> MSVKASGGSSLARPQLYQTVPVSAISQAEQQDRFLEGSELNELTAYFQSGALRLEIAETLTQNADLIVSRAANRIFTGGSPLSYLEKPVERQPALVGASSDSRNGSVTYAESNGSGGLFGGLRSVFSSTGPIPPGFRPINIARYGPSNMQKSLRDMSWFLRYTTYAIVAGDPNIIVVNTRGLKEVIENACSIDATIVAIQEMRAASADYFRNNAQAKEIVLQYFDILLSEFKAPTPANKVRQGPSNDIQGLELPQSYFNAAAKRQKYAMKPGLSALEKNAVIKAAYRQIFERDITKAYSQSISYLESQVRNGDISMKEFVRRLAKSPLYRKQFFEPFINSRALELAFRHILGRGPSSREEVQKYFSIVSSGGLPALVDALVDSQEYADYFGEETVPYLRGLGVEAQECRNWGMQQDLFSYSAPFRKVPQFITTFAQYDRPLPDQHVYGSGNDPLEIQFGAIFPKETRNPSKRPAPFNKDTKRILIHRGPAVNNQVGNPSAVGEFPG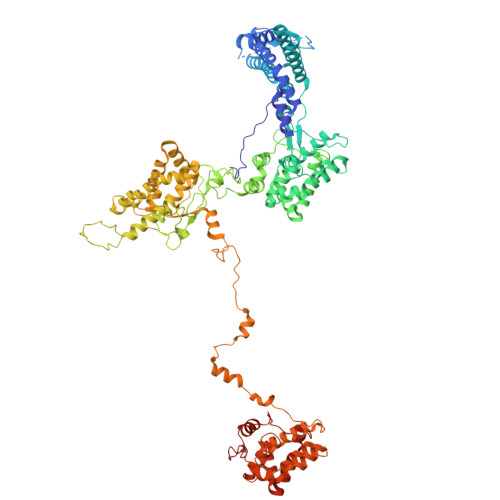SLGAKVFRLNGGLPGAKVGKNTGTSVKFGESSTQALIRAAYRQVFGRDLYEGQRLSVAEIQLENGDISVREFIKRLAKSELFLKLYWAPHYVCKAIEYMHRRLLGRPTYGRQEMNQYFDIASKQGFYAVVEAMIDSKEYSDAFGEDTVPYERYLTPGGLQMRSARVGSLREDIGQRVDKEVTPRFVELGQVSAIRTEPEIAYRSNQGVTRQRQQTKVFKLVSTYDKVAVKNAIRAAYRQVFERDLEPYIINSEFTALESKLSNNEINVKEFIEGLGTSELYMKEFYAPYPNTKVIEMGTKHFLGRAPLNQKEIQQYNQILASQGLKAFIGAMVNGMEYLQTFGEDTVPYRRFPTLPAANFPNTERLYNKLTKQDKELVVPSFTPVVKVGG> MSEEKLGQHYLAALNEAFPGVVLDHAWQTKDQLTVTVKVNYLPEVVEFLYYKQGGWLSVLFGNDERKLNGHYAVYYVLSMEKGHHHHHHHHHHGSTKCWITVRVEVDANKPEYPSVTPRVPAAVWGEREVRDMYGLIPVGLPDERRLVLPDDWPDELYPLRKDSMDYRQRPAPTTDAETYEFINELGDKKNNVVPIGPLHVTSDEPGHFRLFVDGENIIDADYRLFYVHRGMEKLAETRMGYNEVTFLSDRVCGICGFAHSTAYTTSVENAMGIQVPERAQMIRAILLEVERLHSHLLNLGLACHFTGFDSGFMQFFRVRETSMKMAEILTGARKTYGLNLIGGIRRDLLKDDMIQTRQLAQQMRREVQELVDVLLSTPNMEQRTVGIGRLDPEIARDFSNVGPMVRASGHARDTRADHPFVGYGLLPMEVHSEQGCDVISRLKVRINEVYTALNMIDYGLDNLPGGPLMVEGFTYIPHRFALGFAEAPRGDDIHWSMTGD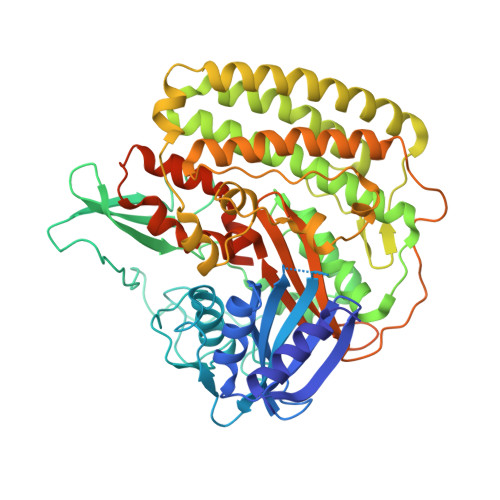NQKLYRWRCRAATYANWPTLRYMLRGNTVSDAPLIIGSLDPCYSCTDRMTVVDVRKKKSKVVPYKELERYSIERKNSPLK>[3x]MGSSHHHHHHSQDPMLEAKFEEASLFKRIIDGFKDCVQLVNFQCKEDGIIAQAVDDSRVLLVSLEIGVEAFQEYRCDHPVTLGMDLTSLSKILRCGNNTDTLTLIADNTPDSIILLFEDTKKDRIAEYSLKLMDIDADFLKIEELQYDSTLSLPSSEFSKIVRDLSQLSDSINIMITKETIKFVADGDIGSGSVI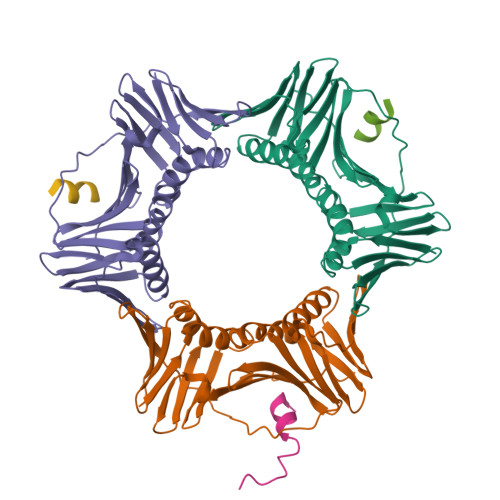IKPFVDMEHPETSIKLEMDQPVDLTFGAKYLLDIIKGSSLSDRVGIRLSSEAPALFQFDLKSGFLQFFLAPKFNDEE;>NGIAAMLQRHSRKRFQL[3x]> ATFEIVNRCSYTVWAAASKGDAALDAGGRQLNSGESWTINVEPGTNGGKIWARTDCYFDDSGSGICKTGDCGGLLRCARFGRPPTTLAEFSLNQYGKDYIDISNIKGFNVPMDFSPTTRGCRGVRCAADIVGQCPAKLKAPGGGCNDACTVFQTSEYCCTTGKCGPTEYSRFFKRLCPDAFSYVLDKPTTVTCPGSSNYRVTFCPTA

Among the sweet-tasting proteins, thaumatin is ~100,000 times sweeter than sucrose on a molar basis and about 1,600 times sweeter on a weight basis. The intensely sweet taste of thaumatin has been widely used not only as a natural sweetener, but also as a flavor enhancer and for masking unpleasant tastes in the food and pharmaceutical industries. Site-directed mutagenesis studies revealed that six lysine residues of Lys19, Lys49, Lys67, Lys106, Lys163, and Lys187, and three arginine residues of Arg76, Arg79, and Arg82 located on the cleft-containing side are responsible for sweetness, and two amino acids residues, Lys67 and Arg82, are particularly important for sweetness. In the present study, three mutant X-ray crystallographic structures of thaumatin (K78A, K106A, and K137A) were determined at resolutions of 1.07, 1.07 and 1.01 Å, respectively.

The final model of the structure of K78A thaumatin consists of a total of 3,284 protein atoms including hydrogen atoms, 20 tartrate atoms, 24 glycerol atoms and 279 water molecules. The threshold values of K78A and K137A were 220 and 230 nM, respectively, and sweetness decreased by ~5-fold when compared to recombinant and plant thaumatin. The B-factors of the main-chain and side-chain of mutated residue Ala78 were 19.64 and 28.49 Å2, respectively. The normalized B-factor ratio (B-factor of residue/Average B-factor) of this residue was 1.63 for main-chain and 1.55 for side-chain. These values were substantially lower than the normalized B-factor ratio of Lys78 of recombinant thaumatin (1.77 for main-chain and 2.20 for side-chain) in which the B-factors of main-chain and side-chain are 17.44 and 31.24 Å2, respectively. The normalized B-factor ratio was reduced 0.65 for side-chain, suggesting that the flexibility of the position of the mutated site of 78 seemed to decrease. Compared to recombinant thaumatin, the blue color of the mutated site of K78A dramatically changed and the volume of the side-chain was almost lost. These results suggested that the distributions and volume of positive charge from lysine residue were substantially reduced. In our interaction model, two flexible residues, i.e., Lys78 and Lys137 interacted with the sweet receptor within 5.0 Å.(2~{R},3~{S},4~{R},5~{R},6~{R})-5-azanyl-2-(hydroxymethyl)-6-(4-phenyl-1~{H}-imidazol-2-yl)oxane-3,4-diol | C15 H19 N3 O4 | 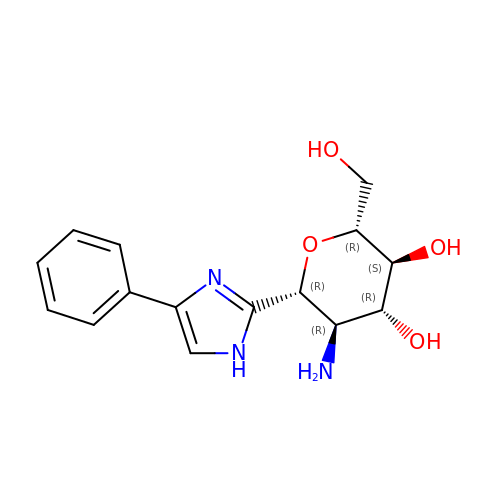XNWVPLWFFIGCKG-DHGKCCLASA-N> VTSYTLNEVVPLKDVVPEWVRIGFSATTGAEFAAHEVHS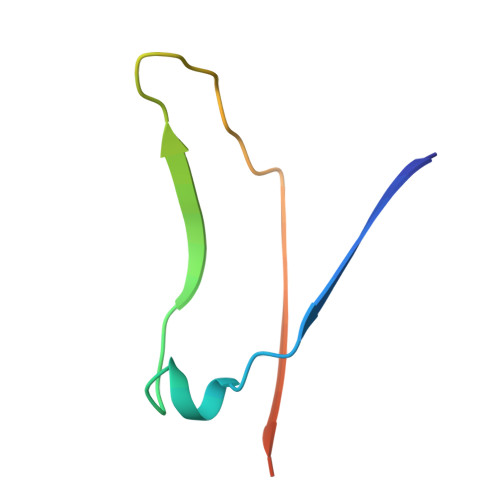WSFHSQLGHTSKS Acetohydroxyacid synthase (AHAS), also known as acetolactate synthase, is the first enzyme of the branched chain amino acid (BCAA) biosynthesis pathway, and is the target for more than 50 of these commercial herbicides. Since the introduction of these herbicides, 197 site-of-action resistance isolates have been identified. These sites are mainly focused on just eight amino acids 1 with all located in the substrate access channel or the catalytic pocket of AHAS. Here, we show that these mutations can have two effects (i) to reduce binding affinity of the herbicides and (ii) to abolish time-dependent accumulative inhibition, critical to the exceptional effectiveness of this class of herbicide.

Next, the crystal structure of the W574L mutant in complex with BS was determined, showing the overall position of BS is unchanged compared to WT AtAHAS. As for CE, the structure revealed that the binding of BS is strongly affected by the loss of π−π interactions when leucine replaces tryptophan. This correlates with the loss of affinity (150-fold), this despite the fact that the two other aromatic rings contained within BS make numerous conserved interactions with the polypeptide the observation that there is only a small increase in B-factors for BS when compared to its binding with the WT enzyme. As for CE, the presence of leucine triggers the rotation of the heterocyclic ring, however, to a lesser extent. Indeed, refinements of the structure with various products (ThThDP vs ThAThDP plus peracetate) suggest that ThDP in this structure is a mixture of ThThDP and ThAThDP/peracetate. In agreement with this, the kinetic data show BS can induce accumulative inhibition in the W574L mutant. The results show that the W574L mutation abolishes accumulative inhibition for all inhibitors except for BS.

> TFISRFAPDQPRKGADILVEALERQGVETVFAYPGGASMEIHQALTRSSSIRNVLPRHEQGGVFAAEGYARSSGKPGICIATSGPGATNLVSGLADALLDSVPLVAITGQVPRRMIGTDAFQETPIVEVTRSITKHNYLVMDVEDIPRIIEEAFFLATSGRPGPVLVDVPKDIQQQLAIPNWEQAMRLPGYMSRMPKPPEDSHLEQIVRLISESKKPVLYVGGGCLNSSDELGRFVELTGIPVASTLMGLGSYPEDDELSLHMLGMHGTVYANYAVEHSDLLLAFGVRFDDRVTGKLEAFASRAKIVHIDIDSAEIGKNKTPHVSVCGDVKLALQGMNKVLENRAEELKLDFGVWRNELNVQKQKFPLSFKTFGEAIPPQYAIKVLDELTDGKAIISTGVGQHQMWAAQFYNYKKPRQWLSSGGLGAMGFGLPAAIGASVANPDAIVVDIDGDGSFIMNVQELATIRVENLPVKVLLLNNQHLGMVMQLEDRFYKANRAHTFLGDPAQEDEIFPNMLLFAAACGIPAARVTKKADLREAIQTMLDTPGPYLLDVICPHQEHVLPMIPSGGTFNDVITEGDGRLEHHHHHH>MTSRDGYQWTPETGLTQGVPSLGVISPPTNIEDTDKDGPWDVIVIGGGYCGLTATRDLTVAGFKTLLLEARDRIGGRSWSSNIDGYPYEMGGTWVHWHQSHVWREITRYKMHNALSPSFNFSRGVNHFQLRTNPTTSTYMTHEAEDELLRSALHKFTNVDGTNGRTVLPFPHDMFYVPEFRKYDEMSYSERIDQIRDELSLNERSSLEALILTCSGGTLENSSFGEFLHWWAMSGYTYQGCQDCLTSYKFKDGQSAFARRFWEEAAGTGRLGYVFGCPVRSVVNERDAARVTARDGREFVAKRVVCTIPLNVLSTIQFSPALSTERISAMQAGHVSMCTKVHAEVDNKDMRSWTGIAYPFNKLCYAIGDGTTPAGNTHLVCFGNSANHIQPDEDVRETLKAVGQLAPGTFGVKRLVF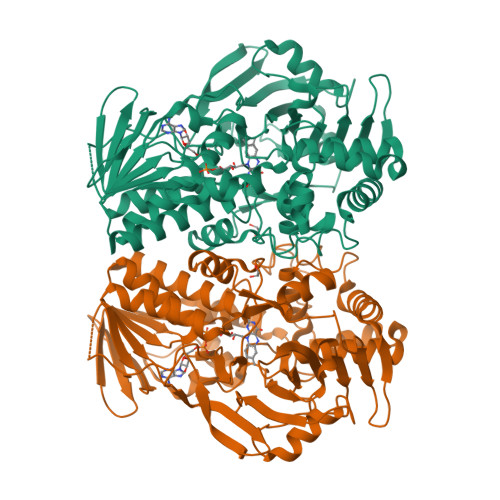HNWVKDEFAKGAGFFSRPGMVSECLQGLREKHGGVVFANSDWALGWRSFIDGAIEEGTRAARVVLEELGTKREVKARL[4x]>[6x]MDKKQVTDLRSELL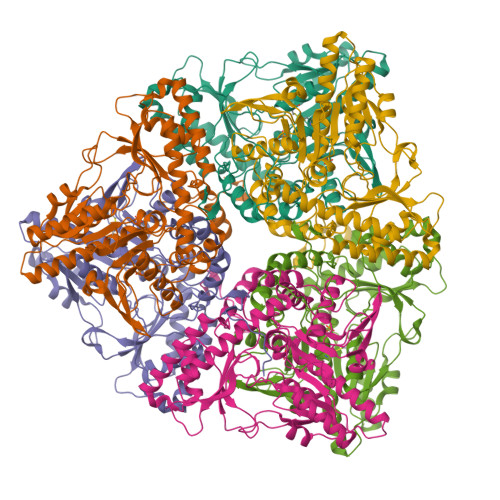DSRFGAKSISTIAESKRFPLHEMRDDVAFQIINDELYLDGNARQNLATFCQTWDDENVHKLMDLSINKNWIDKEEYPQSAAIDLRCVNMVADLWHAPAPKNGQAVGTNTIGSSEACMLGGMAMKWRWRKRMEAAGKPTDKPNLVCGPVQICWHKFARYWDVELREIPMRPGQLFMDPKRMIEACDENTIGVVPTFGVTYTGNYEFPQPLHDALDKFQADTGIDIDMHIDAASGGFLAPFVAPDIVWDFRLPRVKSISASGHKFGLAPLGCGWVIWRDEEALPQELVFNVDYLGGQIGTFAINFSRPAGQVIAQYYEFLRLGREGYTKVQNASYQVAAYLADEIAKLGPYEFICTGRPDEGIPAVCFKLKDGEDPGYTLYDLSERLRLRGWQVPAFTLGGEATDIVVMRIMCRRGFEMDFAELLLEDYKASLKYLSDHPKLQGIAQQNSFKHT> KRAMRRYLERGESIEPLDPSEKANKVLARIFKETELRKLKVLGSGVFGTVHKGVWIPEGESIKIPVCIKVIEDKSGRQSFQAVTDHMLAIGSLDHAHIVRLLGLCPGSSLQLVTQYLPLGSLLDHVRQHRGALGPQLLLNWGVQIAKGMYYLEEHGMVHRNLAARNVLLKSPSQVQVADFGVADLLPPDDKQLLYSEAKTPIKWMALESIHFGKYTHQSDVWSYGVTVWEL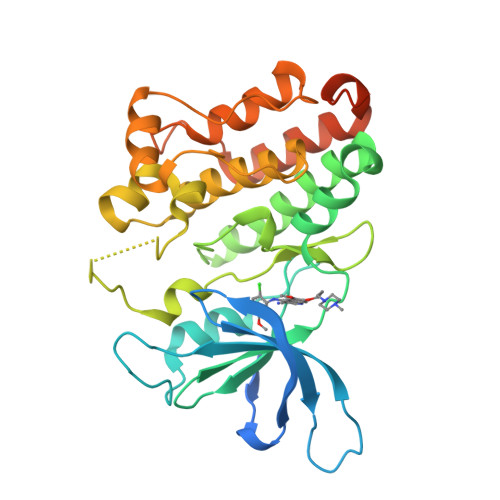MTFGAEPYAGLRLAEVPDLLEKGERLAQPQICTIDVYMVMVKCWMIDENIRPTFKELANEFTRMARDPPRYLVIKRESGPGIAPGPEPHGLTNKKLE>MKLFISPGACSLAPHIALRETGADFEAVKVDLAVRKTEAGEDFLTVNPSGKVPALTLDSGETLTENPAILLYIADQNPASGLAPAEGSLDRYRLLSRLSFLGSEFHKAFVPLFAPATSDEAKAAAAESVKNHLAALDKELAGRDHYAGNAFSVADIYLYVMLGWPAYV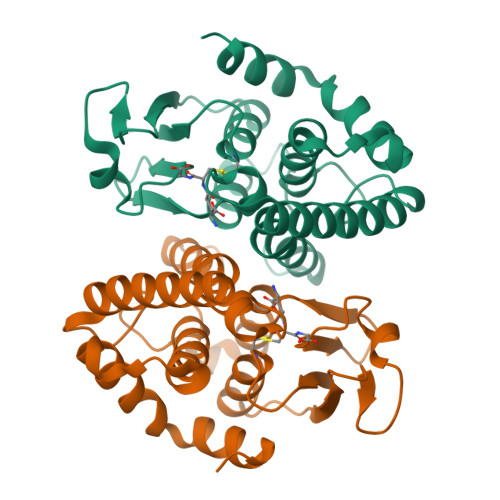GIDMAAYPALGAYAGKIAQRPAVGAALKAEGLA[4x]>[14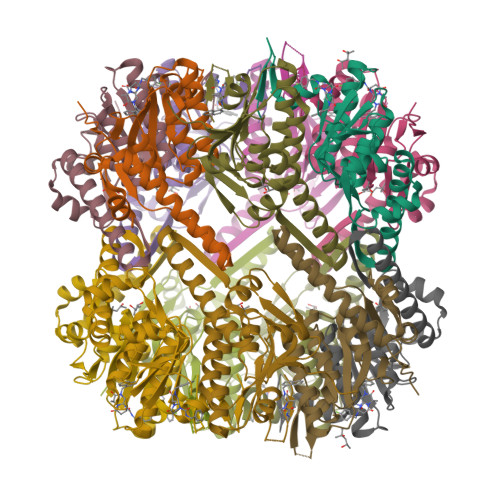x]MNLIPTVIETTNRGERAYDIYSRLLKDRIIMLGSQIDDNVANSIVSQLLFLQAQDSEKDIYLYINSPGGSVTAGFAIYDTIQHIKPDVQTICIGMAASMGSFLLAAGAKGKRFALPNAEVMIHQPLGGAQGQATEIEIAANHILKTREKLNRILSERTGQSIEKIQKDTDRDNFLTAEEAKEYGLIDEVMVPETKLEHHHHHH> PISPIETVPVKLKPGMDGPKVKQWPLTEEKIKALVEICTEMEKEGKISKIGPENPYNTPVFAIKKKDSTKWRKLVDFR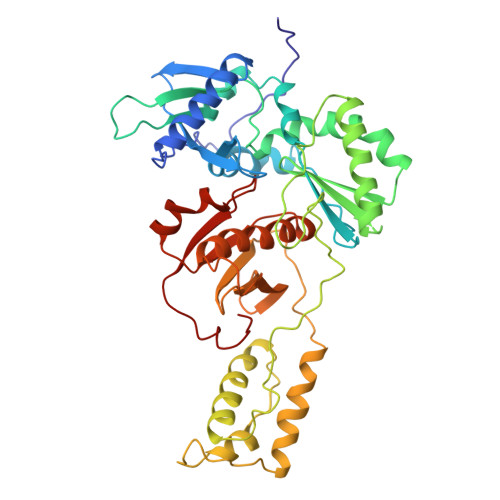ELNKRTQDFWEVQLGIPHPAGLKKKKSVTVLDVGDAYFSVPLDEDFRKYTAFTIPSINNETPGIRYQYNVLPQGWKGSPAIFQSSMTKILEPFKKQNPDIVIYQYMDDLLVGSDLEIGQHRTKIEELRQHLLRWGLTTPDKKHQKEPPFLWMGYELHPDKWTVEPIVLPEKDSWTVNDIQKLVGKLNWASQIYPGIKVRALSKLLRGTKALTEVIPLTEEAELELAENREILKEPVHGVYYDPSKDLIAEIQKQGQGQWTYQIYQEPFKNLKTGKYARMRGAHTNDVKQLTEAVQKITTESIVIWGKTPKFKLPIQKETWETWWTEYWQATWIPEWEFVNTPPLVKLWYQLE>[2x]GPHGEAVVEPEMSNADISDARRGGMLGEPEPLTEKALREASSAIDVLGETLVAEAYCKTWSYREDALLALSKKLMEMPVGTPKEDLKNTLRASVFLVRRAIKDIVTSVFQASLKLLKMIITQYIPKHKLSKLETAHCVERTIPVLLTRTGDSSARLRVTAANFIQEMALFKEVKSLQIIPSYLVQPLKANSSVHLAMSQMGLLARLLKDLGTGSSGFTIDNVMKFSVSALEHRVYEVRETAVRIILDMYRQHQASILEYLPPDDSNTRRNILYKTIFEGFAKIDGRAT

Cep104 is a key factor involved in cilia formation and length regulation that rides on the ends of elongating and shrinking cilia. It is mutated in Joubert syndrome, a genetically heterogeneous ciliopathy. Here we provide structural and biochemical data that Cep104 contains a tubulin-binding TOG (tumor overexpressed gene) domain and a novel C2HC zinc finger array. We have structurally characterized two of these domains, a central tubulin-binding TOG (tumor overexpressed gene) domain and a C-terminal domain consisting of an array of four Zn fingers (ZNF domain).

To this end, we purified recombinant human Cep104 TOG and subjected it to size-exclusion chromatography coupled with multi-angle light scattering (SEC-MALS) in the presence or absence of tubulin. The results shown in Figure 1D and Table 1 demonstrate that Cep104 TOG is indeed a tubulin-binding domain and suggest a probable 1:1 complex between both proteins. To gain a structural insight into the Cep104-tubulin interaction, we determined the high-resolution structure of the TOG domain to a resolution of 2.3 Å by X-ray crystallography. Characteristic for TOG domains, the Cep104 TOG structure consists of six HEAT-like repeats A–F and globally superposes well with other known TOG structures (root-mean-square deviation [rmsd] 3–3.5 Å, Figure S2C). Repeats A–C and E of the Cep104 TOG domain are canonical, whereas repeats D and F are partly distorted. A structure comparison of Cep104 TOG with the TOG domains from XMAP215 and CLASP proteins shows that the conformation of the loops that define their tubulin-binding interface is more conserved than those of the loops found on the opposite side. Furthermore, the residues on that side of the Cep104 TOG domain are highly conserved across different species. Structure superposition of the human Cep104 TOG domain with the Stu2 TOG1 domain in complex with tubulin suggest that key residues implicated in the Stu2-tubulin interaction (Ayaz et al., 2012) are conserved, such as the W448, V493, and R626 residues. To test whether these residues are indeed crucial for tubulin binding, we introduced point mutations in Cep104 TOG, produced the corresponding recombinant proteins, and subjected them to SEC-MALS in the presence or absence of tubulin. The results shown in Figure 1D and Table 1 demonstrate that these mutants are indeed severely (V493D and R626A) or mildly (W448A) impaired in their ability to interact with tubulin. Thus, the Cep104 TOG domain engages tubulin in a similar way to the Stu2 TOG1 domain. Tubulin-binding TOG domains, e.g., in the XMAP215 family of MAPs, act to stabilize microtubules through facilitating tubulin addition to microtubule ends, and we speculate that the TOG domain in Cep104 has an analogous role.>MPQDVDFHIPLPGRQSPDHARAEAEQLAWPRSLGLIRSDAAAERHLRGGYADLASRFYPHATGADLDLGVDLMSWFFLFDDLFDGPRGENPEDTKQLTDQVAAALDGPLPDTAPPIAHGFADIWRRTCEGMTPAWCARSARHWRNYFDGYVDEAESRFWNAPCDSAAQYLAMRRHTIGVQPTVDLAERAGRFE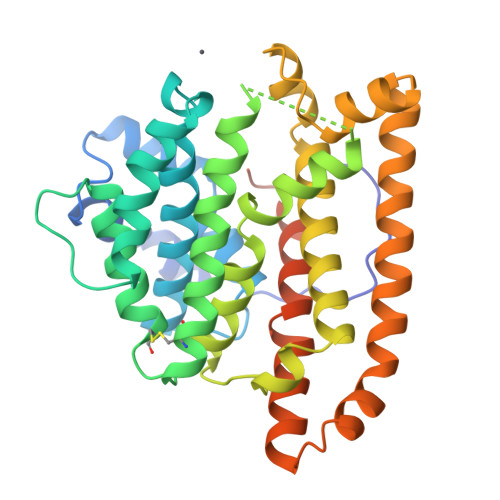VPHRVFDSAVMSAMLQIAVDVNLLLNDIASLEKEEARGEQNNMVMILRREHGWSKSRSVSHMQNEVRARLEQYLLLESCLPKVGEIYQLDTAEREALERYRTDAVRTVIRGSYDWHRSSGRYDAEFALAAGAQGYLEELGSSAH[2x]2-keto 3 deoxy 6 phospho gluconate | C6 H11 O9 P | 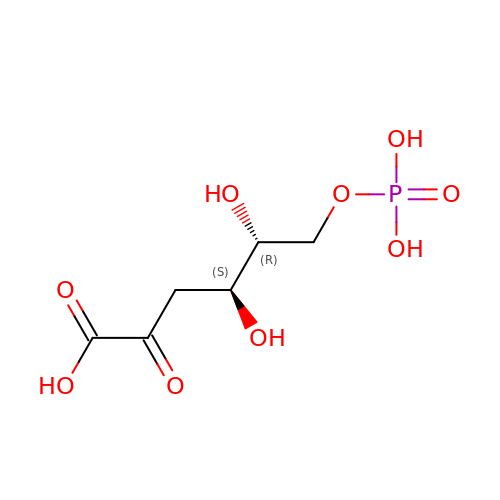OVPRPPOVAXRCED-WVZVXSGGSA-N Noroviruses infect a plethora of animal species, including humans, dogs, and bats. One such group is GX bat noroviruses (1–3), which remain poorly understood but are gaining interest due to bats’ roles as reservoirs for zoonotic viruses. Indeed, a recent study showed that bat noroviruses bind histo-blood group antigens (HBGAs), which are co-factors for human noroviruses. In this study, we observe novel structural factors on a GX bat norovirus (NPIH26) capsid that restrict HBGA binding and demonstrate that an emerging genotype, GII.27 binds an HBGA at a common pocket using X-ray crystallography.

In the case of GII.27, we obtained X-ray data showing that a single A-trisaccharide molecule bound to the P domain dimer, as previously observed with other GII genotypes. P domain and A-trisaccharide binding interaction was mediated by a network of hydrogen bonds, a hydrophobic interaction, and several water-mediated interactions by both P domain monomers, which was observed with other GII genotypes. The electron density of the bound fucose and A-trisaccharide molecules was clearly discernible and modeled during the final refinement. Overall, NPIH26 norovirus exhibited a divergent fucose binding site from human norovirus and had structural constraints for binding HBGAs, whereas the GII.27 norovirus bound an A-trisaccharide at the common GII HBGA pocket.

>[2x]SKPFTIPILTIGEMTNSRFPVAIDMLHTSPTDNFIVQPQNGRCTLDGELQGTTQLVASNICAFRGSISGHENNGDQHQWHFSITNPNGTPFDPTEDVPAPLGTPDFKGQLYGVISQRNREGSSGNGNQKANRSHEGVISTVAPRFTPKLGSVMIGTWTTDDIQDQPSRFTPVGLNDDDNYKQWELPNYSGALTLNMGLAPSVFPTYPGEQLLFFRSYIPMKGGYGSPYIDCLIPQEWISHFYQESAPSQTDVALIRYVNPDTGRVLFEAKLHRQGYITVAKTGDSPINVPANGYFRFDSWVSQFYSLAPM>[8x]MMVISEKVRKALNEQLNREIYSSYLYLSMATYFDAEGFKGFAHWMKKQAQEELTHAMKFYEYIYERGGR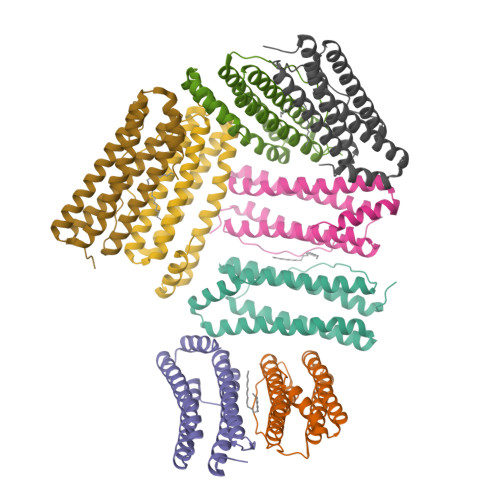VELEAIEKPPSNWNGIKDAFEAALKHEEFVTQSIYNILELASEEKDHATVSFLKWFVDEQVEEEDQVREILDLLEKANGQMSVIFQLDRYLGQRE>MAIERTLSIVKPDAVSKNHIGEIFARFEKAGLKIVATKMKHLSQ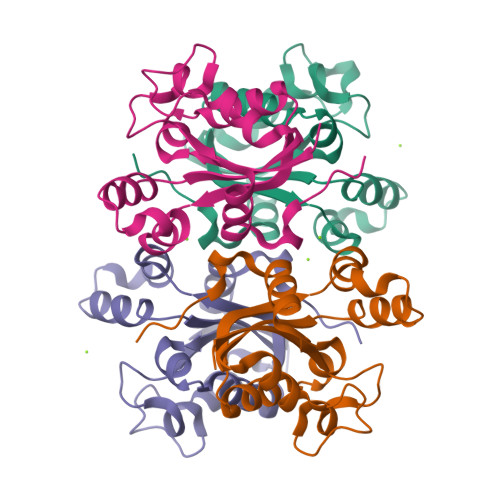ADAEGFYAEHKERGFFGDLVAFMTSGPVVVSVLEGENAVLAHREILGATNPKEAAPGTIRADFAVSIDENAAHGSDSVASAEREIAYFFADNEICPRTR[4x]> MKRRFTLLGSVVALALSSTALASDAPASRGCADDAGWNDPAMPQKVYGNTWYVGTCGISALLVTSDAGHILVDAATPQAGPQILANIRALGFRPEDVRAIVLSHEHFDHAGSLAELQKATGAPVYARAPAIDTLKRGLPDRTDPQFEVAEPVAPVANIVTLADDGVVSVGPLALTAVASPGHTPGGTSWTWRSCEGDDCRQMVYADSLTAISDDVYRYS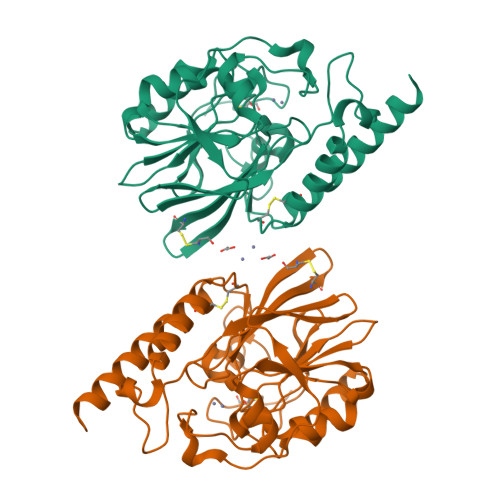DDAAHPGYLAAFRNTLARVAALDCDILVTPHPSASGLWNRIGPRAAAPLMDTTACRRYAQGARQRLEKRLAEEAAA>MVANPEHYIKHPLQNRWALWFFKNDKSKTWQANLRLISKFDTVEDFWALYNHIQLSSNLMPGCDYSLFKDGIEPMWEDEKNKRGGRWLITLNKQQRRSDLDRFWLETLLCLIGESFDDYSDDVCGAVVNVRAKGDKIA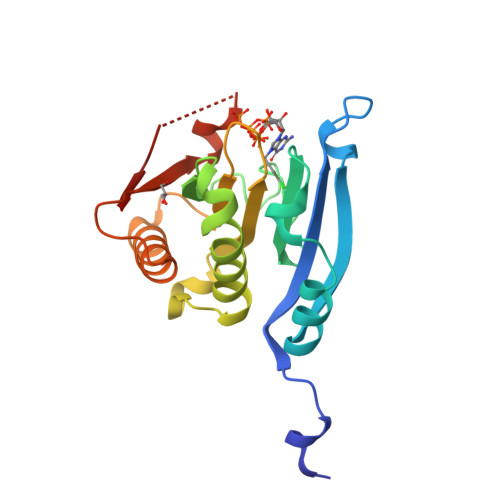IWTTECENRDAVTHIGRVYKERLGLPPKIVIGYQSHADTATKSGSTTKNRFVV[4x]The membrane protein FlhB is a highly conserved component of the flagellar secretion system. It is composed of an N-­terminal transmembrane domain and a C-terminal cytoplasmic domain (FlhBC). Flagellar FlhBC consists of a globular domain composed of a four-stranded β-sheet surrounded by four α-helices. The globular domain is preceded by a long N-terminal α-helix (α1) that connects the cytoplasmic globular part of FlhB to the transmembrane domain.

In the case of SalFlhBC the final model comprises residues 229–353 out of 219–383 in the crystallized protein, with a cleavage after Asn269. No electron density was observed for residues 219–228 and 354–383. Zn2+ was added to the crystallization solution and was necessary to obtain well diffracting crystals. In the model of SalFlhBC helix α1 is longer and has a kink at the highly conserved residue Gly236. Although the kink may arise from the crystal packing, our data show potential flexibility of the linker around this conserved glycine residue. However, these additional residues (residues 354–383) were not visible in the electron-density map, suggesting that they are unfolded. This region in SalFlhB is rich in proline residues, making it unlikely to form any stable structure. In the SalFlhBC crystal α1 primarily contacts α1 and α2 of adjacent molecules, while in the AquFlhBC crystal α1 primarily contacts α4 and the cleavage site between β1 and β2. Molecular-dynamics calculations demonstrate that the linker region is the most flexible part of FlhBC and that the deletion of the loop reduces this flexibility.

> MKLRMSRQDIRDEFKESEGDPHVKGKIRQMQRAAAQRRMMEDVPKADVIVTN;> PTHYSVALQYDENKMSAPKVVAKGAGLIALRIREIGAEHRVPTLEAPPLARALYRHAEIGQQIPGQLYAAVAEVLAWVWQLKRWRLAGGQRPPQPENLPVPEALDFMNEKNTDA6-amino-4-{2-[(cyclohexylmethyl)amino]ethyl}-2-[(2-phenylethyl)amino]-3,7-dihydro-8H-imidazo[4,5-g]quinazolin-8-one | C26 H33 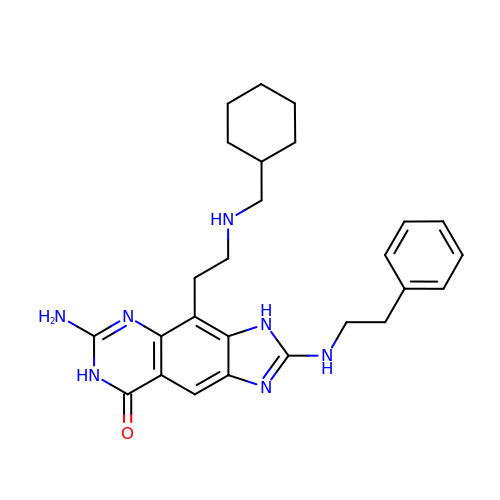N7 O | MTBBEHDSALYQRB-UHFFFAOYSA-N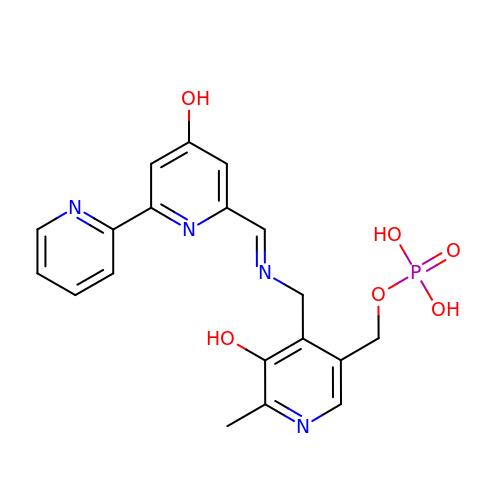[5-hydroxy-4-({(E)-[(4-hydroxy-2,2'-bipyridin-6-yl)methylidene]amino}methyl)-6-methylpyridin-3-yl]methyl dihydrogen phosphate | C19 H19 N4 O6 P | MXRNEZXMCIDZEM-AWQFTUOYSA-N> DYSNPGHHPPRHN;> CNWTGVKCNRRGEVSEIQLKEKQLQGSLPVTSLRSLKSLTSLTLSSLQLTGVIPKEIGDFTELELLDLSDNSLSGDIPVEIFRLKKLKTLSLNTNNLEGHIPMEIGNLSGLVELMLFDNKLSGEIPRSIGELKNLQVLRAGGNKNLRGELPWEIGNCENLVMLGLAETSLSGKLPASIGNLKRVQTIAIYTSLLSGPIPDEIGYCTELQNLYLYQNSISGSIPTTIGGLKKLQSLLLWQNNLVGKIP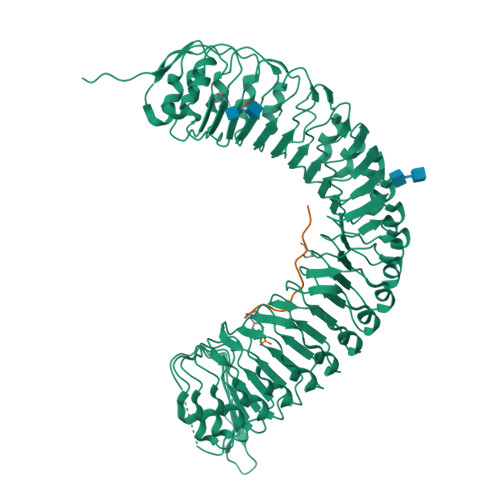TELGNCPELWLIDFSENLLTGTIPRSFGKLENLQELQLSVNQISGTIPEELTNCTKLTHLEIDNNLITGEIPSLMSNLRSLTMFFAWQNKLTGNIPQSLSQCRELQAIDLSYNSLSGSIPKEIFGLRNLTKLLLLSNDLSGFIPPDIGNCTNLYRLRLNGNRLAGSIPSEIGNLKNLNFVDISENRLVGSIPPAISGCESLEFLDLHTNSLSGSLLGTTLPKSLKFIDFSDNALSSTLPPGIGLLTELTKLNLAKNRLSGEIPREISTCRSLQLLNLGENDFSGEIPDELGQIPSLAISLNLSCNRFVGEIPSRFSDLKNLGVLDVSHNQLTGNLNVLTDLQNLVSLNISYNDFSGDLPNTPFFRRLPLSDLASNRGLYISNAIST Retaining α-glucosidases employ a conserved two-step Koshland double displacement mechanism, in which α-glucosidase substrates are hydrolyzed using two key carboxylic acid residues functioning as the catalytic nucleophile (Asp518 in GAA and Asp412 in CjAgd31B, a bacterial homologue of GAA) and catalytic acid/base (Asp616 in GAA and Asp480 in CjAgd31B). Mutations in the gene encoding for GAA can lead to enzyme deficiency which generates multiple phenotypic forms of the lysosomal storage disorder (LSD) Pompe disease (PD). Herein, we report a 1,6-epi-cyclophellitol cyclosulfamidate as a new class of reversible α-glucosidase inhibitors that displays enzyme inhibitory activity by virtue of its conformational mimicry of the substrate when bound in the Michaelis complex.

The X-ray structure of human α-glucosidase rhGAA in complex with sulfamidate 4 revealed that it binds the enzyme active site adopting a 4C1 Michaelis-type conformation in a noncovalent manner. The interactions of the cyclitol moiety of sulfamidate 4 with rhGAA are virtually identical to those observed in previous reported complex structures of rhGAA with the GAA inhibitors, acarbose, 1-deoxynojirimycin (DNJ), and N-hydroxyethyl-DNJ (NHE-DNJ),21 notably with Arg600, His674, Asp404, and the acid/base Asp616, strengthened by solvent-mediated interactions with Asp443, Asp616, Asp645, and Trp481. The endocyclic nitrogen of the sulfamidate moiety establishes a tight hydrogen-bonding interaction with the acid/base Asp616, providing a structural rational for the lack of inhibition of the methylated analogue 5 due to steric hindrance. The endocyclic nitrogen and the sulfate moieties of sulfamidate 4 overlap spatially with the nitrogen and subsite +1 aglycone atomic features, respectively, of acarvosine reported previously, reinforcing that sulfamidate 4 is a true substrate Michaelis complex mimetic for GAA. Methylated analogue 5 proved to be a much weaker inhibitor toward α-glucosidase GAA (IC50 = 485 μM) and inactive toward GANAB, suggesting that there is no room for functionalization at the endocyclic nitrogen. Cyclosulfamidate 4 proved to be a low-micromolar inhibitor of GAA (IC50 = 5.17 μM) and is 5 times more potent than NB-DNJ 2 (IC50 = 26.7 μM). Kinetic parameters determined with increasing 4-MU-α-glucoside concentrations proved that cyclosulfamidate 4 reversibly inhibits GAA with a Ki of 3.40 μM, approximately 5-fold more potent than NB-DNJ 2 (Ki 15.2 μM). Thermostability assays (TSAs) showed that α-glc-cyclosulfamidate 4 stabilizes rhGAA with a maximum shift in inflection temperature (ΔTimax) of 11.2 °C and a half maximal effective concentration (EC50) of 1.16 μM, whereas α-glc-cyclosulfamidate 6 does not prevent enzyme unfolding at increasing temperature. In conclusion, 1,6-epi-cyclophellitol cyclosulfamidate 4 is a selective reversible α-glucosidase ligand that binds through 4C1 conformational Michaelis complex mimicry.

>[2x]QCDVPPNSRFDCAPDKAITQEQCEARGCCYIPAKQGLQGAQMGQPWCFFPPSYPSYKLENLSSSEMGYTATLTRTTPTFFPKDILTLRLDVMMETENRLHFTIKDPANRRYEVPLETPRVHSRAPSPLYSVEFSEEPFGVIVHRQLDGRVLLNTTVAPLFFADQFLQLSTSLPSQYITGLAEHLSPLMLSTSWTRITLWNRDLAPTPGANLYGSHPFYLALEDGGSAHGVFLLNSNAMDVVLQPSPALSWRSTGGILDVYIFLGPEPKSVVQQYLDVVGYPFMPPYWGLGFHLCRWGYSSTAITRQVVENMTRAHFPLDVQWNDLDYMDSRRDFTFNKDGFRDFPAMVQELHQGGRRYMMIVDPAISSSGPAGSYRPYDEGLRRGVFITNETGQPLIGKVWPGSTAFPDFTNPTALAWWEDMVAEFHDQVPFDGMWIDMNEPSNFIRGSEDGCPNNELENPPYVPGVVGGTLQAATICASSHQFLSTHYNLHNLYGLTEAIASHRALVKARGTRPFVISRSTFAGHGRYAGHWTGDVWSSWEQLASSVPEILQFNLLGVPLVGADVCGFLGNTSEELCVRWTQLGAFYPFMRNHNSLLSLPQEPYSFSEPAQQAMRKALTLRYALLPHLYTLFHQAHVAGETVARPLFLEFPKDSSTWTVDHQLLWGEALLITPVLQAGKAEVTGYFPLGTWYDLQTVPIEALGSLPPPPAAPREPAIHSEGQWVTLPAPLDTINVHLRAGYIIPLQGPGLTTTESRQQPMALAVALTKGGEARGELFWDDGESLEVLERGAYTQVIFLARNNTIVNELVRVTSEGAGLQLQKVTVLGVATAPQQVLSNGVPVSNFTYSPDTKVLDICVSLLMGEQFLVSWC>GSEDFTFDGTKRLSVNYVKGILQPTDTCDIWDKIWNFQAKPDDLLISTYPKAGTTWTQEIVELIQNEGDVEKSKRAPTHQRFPFLEMKIPSLGSGLEQAHAMPSPRILKTHLPFHLLPPSLLEKNCKIIYVARNPKDNMVSYYHFQRMNKALPAPGTWEEYFETFLAGKVCWGSWHEHVKGWWEAKDKHRILYLFYEDMKKNPKHEIQKLAEFIGKKLDDKVLDKIVHYTSFDVMKQNPMANYSSIPAEIMDHSISPFMRKGAVGDWKKHFTVAQNERFDEDYKKKMTDTRLTFHFQF[2x]

Cytosolic sulfotransferases (SULTs) comprise a family of enzymes that catalyze the transfer of a sulfonate group from 3′-phosphoadenosine 5′-phosphosulfate (PAPS) to an acceptor group of the substrate. In doing so, SULTs modulate the activities of a large array of small endogenous and foreign chemicals, including drugs, toxic compounds, steroid hormones, and neurotransmitters. As expected, all SULTs share the same basic fold: a central four-stranded parallel β-sheet surrounded by α-helices and three loops that are often disordered (dashed lines) in the absence of PAP and/or substrate. The crystal structures of SULT1C3 bound to PAP, apo SULT1C2, a ternary complex of SULT1C2 bound to PAP, and the environmental toxin, pentachlorophenol (PCP), and SULT4A1 were solved at 3.2, 2.0, 1.8, and 2.2 Å, respectively.

In order to better understand the mechanism of inhibition by PCP, we determined the structure of SULT1C2 bound to PAP and PCP. The structure reveals that the protein undergoes a disorder–order transition upon PCP and PAP binding. Helices α4, α5, and αı5, and loops α5-α6 and α15-α16 are ordered only in the ternary complex, but not in the apo SULT1C2 structure. PCP is found in the substrate binding pocket and therefore appears to be a competitive inhibitor, consistent with crystallographic analysis of SULT1E1 bound to PAP and 3,5,3′,5′-tetrachlorobiphenol. Comparison of the SULT1C2-PAP-PCP and SULT1E1-PAP-estradiol structures revealed two structural features that may be relevant in explaining the mechanism of PCP inhibition. In the co-crystal structures, the phenol moieties of PCP and estradiol share the same relative position and orientation, positioning the phenolic OH within hydrogen-bond distance of the catalytic histidine. Our structure shows that PCP appears to be in a catalytically competent conformation. However, PCP and estradiol differ dramatically in the acidity of their hydroxyl groups; the estimated pKa for estradiol is approximately 15, whereas that for PCP is 4.5. Thus, although PCP appears to bind in a catalytically competent conformation, the phenolic oxygen of PCP may be too weak a nucleophile to attack the sulfonate of PAPS. Although steric and conformational factors clearly play a role, our structure of SULT1C2 with PCP and PAP suggests a key role for the electronic nature of the halogenated phenols.5-[1-[(1S)-1-(4-fluorophenyl)ethyl]-[1,2,3]triazolo[4,5-c]quinolin-8-yl]-1,3-benzoxazole | C24 H16 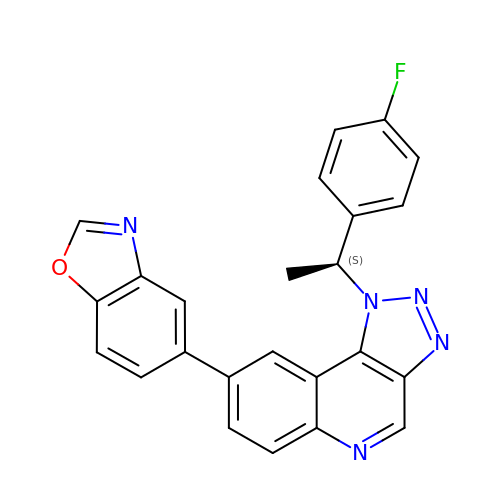F N5 O | BHKVSOQUPYXVRZ-AWEZNQCLSA-N> AP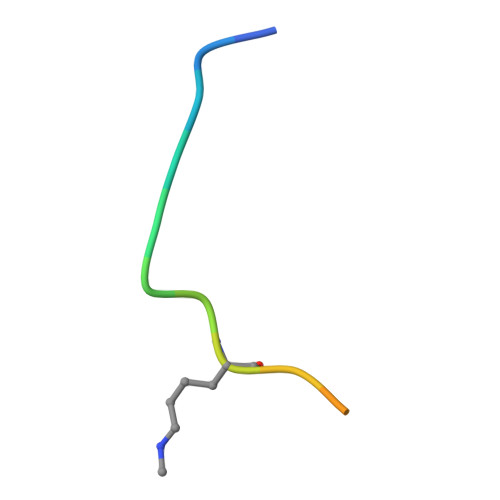ATGGVKKPHRYRP N-(1,2-oxazol-3-yl)-2-phenylacetamide | C11 H10 N2 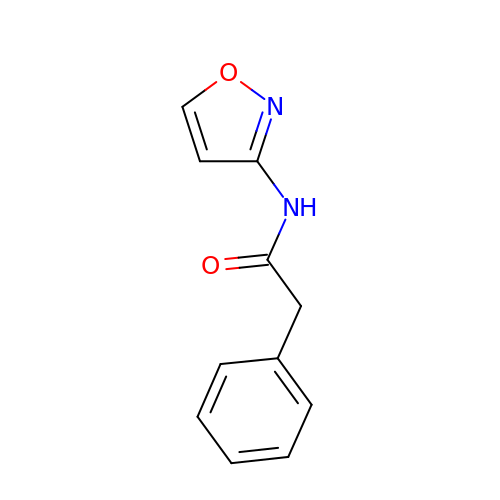O2 | SGBROXCJKREELC-UHFFFAOYSA-N>[6x]GAMGSSSVWGVAFSPDGQTIASASDDKTVKLWNRNGQLLQTLTGHSSSVWGVAFSPDGQTIASASD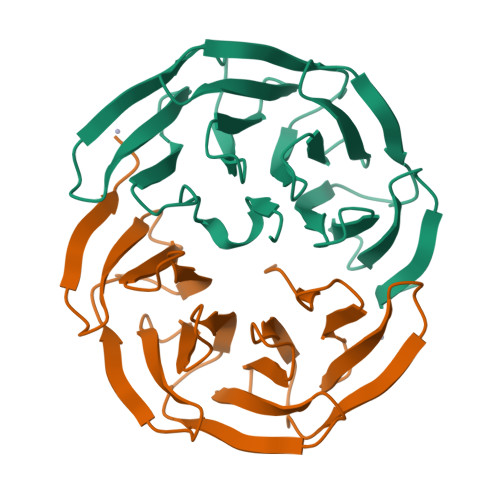DKTVKLWNRNGQLLQTLTGHSSSVWGVAFSPDGQTIASASDDKTVKLWNRNGQLLQTLTGHSSSVWGVAFSPDGQTIASASDDKTVKLWNRNGQLLQTLTGH> MTSLYAPGAEDIRQRLRPFGFFFEKSLKDLIKGIRSHNETPEKLDQFFKQVLSECREEVNSPDLNSKTNAVLKLTYLEMYGFDMAWCNFHILEVMSSNKLQQKRVGYLAASQSFYKDSDILMLATNLLKKDLKYDGNNDVVKVGIALSGLSTIITPSLARDIADDLFTMLNSTRPYIRKKAITALFKVFLQYPEALRDNFDKFVSKLDDDDISVVSAAVSVICELSKKNPQPFIQLSPLLYEILVTIDNNWIIIRLLKLFTNLSQVEPKLRAKLLPKILELMESTVATSVIYESVNCIVKGNMLEEDDFETAMACLERLHTFCDSQDPNLRYISCILFYKIGKINTDFISRFDQLIIRLLSDVDVSIRSKAIELVEGIVDEDNLKAIVQTLMKQFVDEDVVILQTGSIVYEKSKRIPIIIPENYKIKMVNVIISICSADNYSSVNDFEWYNAVIMDLAMLCQDISDKSLGSKIGEQFRNLMIKVPSMREVTIANIIKLISNDNINKQLPTVLRECIWCLGEFSTLVENGNDLIKIMTENISYYSHSVQEVLILALVKVFSNWCNNFQEDKRFEIKMVLKELIEFFENLSYSSTFEVQERSVEVLEFLRLSLEALEEDTEGLPMLLSEVLPSFFNAYELAPIARGTQLKLAVDENLDLETPFLTKEAADELLDEQKSDAISDLMSDISMDEQVELKFVDDSDTSYEEKEKLDDFENPFEIEREKERMSNPYYLGEEDEERTKNSKDLLDLNEEESSDKKPETIRLNRTDNSLNSLSLSTTEISRKKKKGKKKNRVQVLSDEPVIEAAPKRKDAFQKPHDNHSTQNPLKKDKINLRMHSQLENFDFSNFGQSSNAGRGSQEEGNLRKEDELELSRLEANLIVKDEKDNLSDTEEVIVIKKKKKGKKSKSKNKLKTKAKNSPEPNEFLRDQSTDIRTLQVDGSDYKDDDDKDYKDDDDKDYKDDDDK;> MVDSIHRIASALDTAKVITREAAAVATSKLGESSYTYYSQNINPQQLVTLLNSRNSREVRDAMKRIISIMASDDDSIDVQLYFADVVKNITTNDTKVKRLIHLYLLRFAENDPNLTLLSINSLQKSLSDSNSELRCFALSALSDMKMSSLAPIILHTVKKLVTDPSAMVRGEVALAIIKLYRAGKNDYHEELLDILKELMADTDPKVISCAVLAYKECYADHLELLHGHFRRYCRIIKQLDSWSQSYLIELLIKYCKQYLPKPTVVDKSSEGSPRSCPLPDKYNEIEYPSYEVVNDPDLDLFLQSLNCLIYSSNPTVILSCCNALYQLASPLQMKNTKFIEALVRTVTMTENQGNKEMLLQAIHFLSILDQTLFLPYTKKFYVFPKDPIVASIWKIQILSTLINESNVKEIFKELKYYVASAHFPENVVIMAVKSLSRCGQLSTSWESHVMKWLIDHMESHNLSASVLDAYVNVIRMLVQKNPTKHLRIIFKLADLLTVQTSLADNARAGIVWLFGEIASIEFKICPDVLRRLIQNFSNEGPETRCQILVLSAKLLSYDIDNFKQAQVTGSEENNQNPPYYDFSGSRISQMYNAVLYLAKYDDEFDIRDRARMISSLFDSGKYEIVSLLLQAPKPTARSDDFIVSARLETHTPEIKEFFRMLPWNTEITEVGETGNDIREGAELKDYNKYKKSFSSQSFITNNSARSFTSSSNAKLTGINDGDSNSISGKGNVNTFTSQNGKKYRLQSLDEFFSDIPERKSKPRKIIKVVEESSDEDEDESEESSDDDEYSDSSLGTSSSGTSSSHLEL;> MYLSFYITDTKNKLIFQYLLGATAPSFKHLWTRVQSTCPQLLEDSSSDDYLDHSMVGRDLEVYKYFSVINKLNYWCLASTSKSKGPLDCFTFLETIDRILLEYFDKDKLSIKKIVNNYDRISLIFNCCVEAGEPNVSDMLYVNKIKEAVPERSDLSKFISSTAHNLQQAVQLPQQRQQQLQQNQISRGSNSLIENEEIVPWRTSRASKHENNELYVDLLETFHVVFEKKKSHLRLLTGSIHGIVDVRSYLNDNPLVAVKLNTMGNDIGIPSLHDCVEINDGVFSPSNITFIPPDGKFRLLEYSVDLSSQVKQSGVRMNSIGLMSLHFQNGLGKDSDEFELSLNIENFKKVSQVDDLKIDLQFNVENADPNEIAYKIKILRNTHGRFENSIIMGQGQWIFDKSTATGTVPVLRGCIEYENTGPNFTKKVDLQTVSLEYSYIGQSASGIYVEAIDIVSGLTIGKNTKLYKGAKYKTQTGNFQVRL;> MIHAVLIFNKKCQPRLVKFYTPVDLPKQKLLLEQVYELISQRNSDFQSSFLVTPPSLLLSNENNNDEVNNEDIQIIYKNYATLYFTFIVDDQESELAILDLIQTFVESLDRCFTEVNELDLIFNWQTLESVLEEIVQGGMVIETNVNRIVASVDELNKAAESTDSKIGRLTSTGFGSALQAFAQGGFAQWATGQ

Heterotetrameric adapter protein (AP) complexes are required at several endomembranes for cargo binding. Finally, AP-3 functions between the trans Golgi and the vacuole in yeast, whereas mammalian AP-3 localizes to a tubular endosomal compartment, in addition to or instead of the TGN. Here we present cryo-EM structures of the full-length stable 300 kDa yeast AP-3 complex. The structures reveal that AP-3 adopts an open conformation in solution, comparable to the membrane-bound conformations of AP-1 or AP-2.

We selected three classes, which showed the most distinct conformational differences based on the gap created between the N-Apl5 and C-Apm3 subunits as well as the overall length of the AP-3 complex in the 2D class averages and the 3D reconstructions. Indeed, the overall length of the AP-3 complex varied from 11.5 nm in its most compact to 13 nm in its stretched form. Similarly, the distance between the N-Apl5 and C-Apm3 subunits increases from ∼2.2 nm to ∼3.9 nm, demonstrating the variability of the “open” AP-3 complex in solution. The large α-solenoid domains of Apl5 and Apl6 contain several hinge regions that allow an accordion-like expansion and partial rotation of the domains. The general organization of both the compact and stretched conformation of the yeast AP-3 complex is similar to that of mammalian AP-1 and AP-2. A direct comparison with the open and closed conformation of AP-1 revealed that both conformations of AP-3 represent a more open state of adaptor proteins than previously observed for membrane-bound AP-1 or AP-2, in which the N-terminal region of Apl5 is rotated ∼31° (compact) and ∼38° (stretched) upward and tilted away from the core of the complex.1,3-DI(N-PROPYLOXY-A-MANNOPYRANOSYL)-CARBOMYL 5-METHYAZIDO-BENZENE 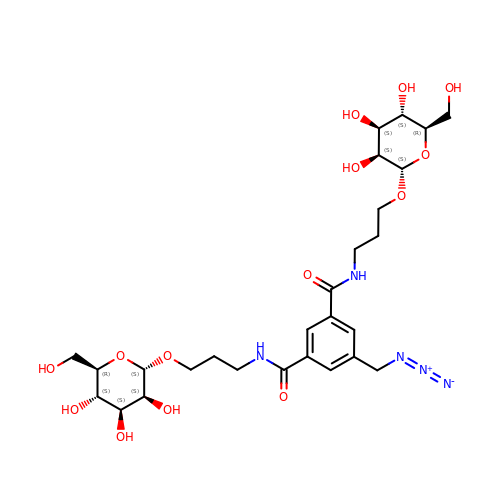| C27 H41 N5 O14 | GKRIMQPDERYOML-LHMXEDMUSA-N> AHMGIQRPTSTTTDKKEIKAYLKQVDKIKDDEEPIKTVGKKI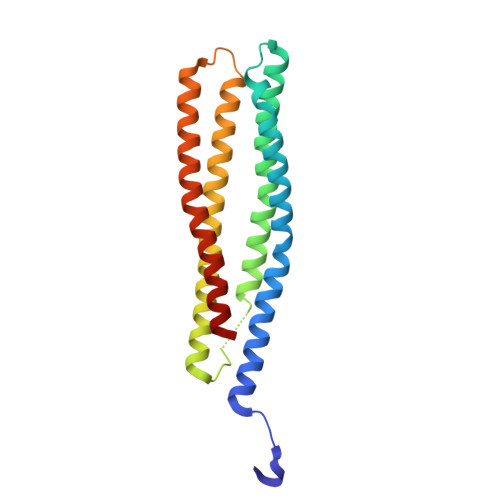AELDEKKKKLTEDVNSKDTAVRGKAVKDLIKNADDRLKEFEKEEDAIKKSEQDFKKAKSHVDNIDNDVKRKEVKQLDDVLKEKYKLHSDYAKAYKKAVNSEKTLFKYLNQNDATQQGVNEKSKAIEQNYKKLKEVSDKYTKVLNKVQKEKQDVDQFK> MRRRSRMLLCFAFLWVLGIAYYMYSGGGSALAGGAGGGAGRKEDWNEIDPIKKKDLHHSNGEEKAQSMETLPPGKVRWPDFNQEAYVGGTMVRSGQDPYARNKFNQVESDKLRMDRAIPDTRHDQCQRKQWRVDLPATSVVITFHNEARSALLRTVVSVLKKSPPHLIKEIILVDDYSNDPEDGALLGKIEKVRVLRNDRREGLMRSRVRGADAAQAKVLTFLDSHCECNEHWLEPLLERVAEDRTRVVSPIIDVINMDNFQYVGASADLKGGFDWNLVFKWDYMTPEQRRSRQGNPVAPIKTPMIAGGLFVMDKFYFEELGKYDMMMDVWGGENLEISFRVWQCGGSLEIIPCSRVGHVFRKQHPYTFPGGSGTVFARNTRRAAEVWMDEYKNFYYAAVPSARNVPYGNIQSRLELRKKLSCKPFKWYLENVYPELRVPDHQDIAFGALQQGTNCLDTLGHFADGVVGVYECHNAGGNQEWALTKEKSVKHMDLCLTVVDRAPGSLIKLQGCREDDSRQKWEQIEGNSKLRHVGSN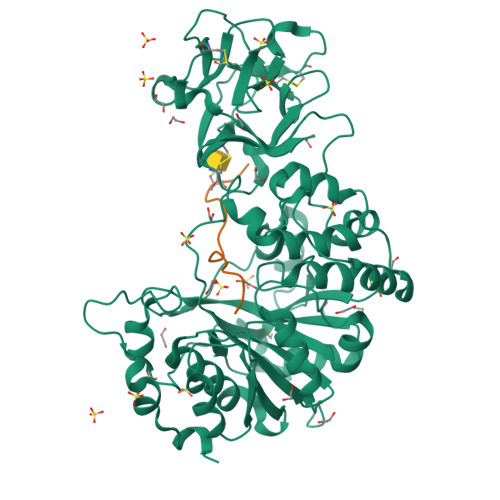LCLDSRTAKSGGLSVEVCGPALSQQWKFTLNLQQ;> GTTPSPVPTTSTCSAA> GPLGSTEVLCLMNMVLPEELLDDEEYEEIVEDVRDECSKYGLVKSIEIPRPVDGVEVPGCGKIFVEFTSVFDCQKAMQGLTGRKFANRVVVTKYCD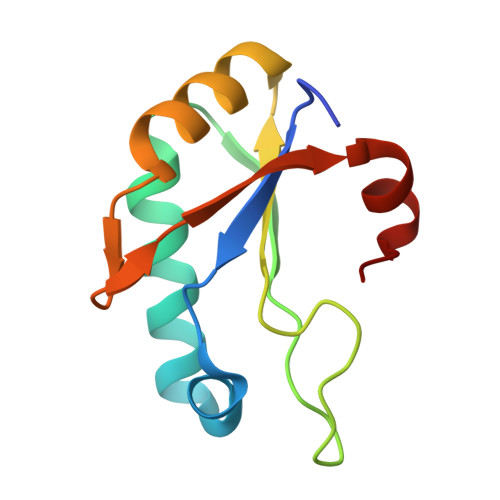PDSYHRRDFW>MGHQNAAVSENQNHDDGAASSPGFKLVGFSKFVRKNPKSDKFKVKRFHHIEFWCGDATNVARRFSWGLGMRFSAKSDLSTGNMVHASYLLTSGDLRFLFTAPYSPSLSAGEIKPTTTASIPSFDHGSCRSFFSSHGLGVRAVAIEVEDAESAFSISVANGAIPSSPPIVLNEAVTIAEVKLYGDVVLRYVSYKAEDTEKSEFLPGFERVEDASSFPLDYGIRRLDHAVGNVPELGPALTYVAGFTGFHQFAEFTADDVGTAESGLNSAVLASNDEMVLLPINEPVHGTKRKSQIQTYLEHNEGAGLQHLALMSEDIFRTLREMRKRSSIGGFDFMPSPPPTYYQNLKKRVGDVLSDDQIKECEELGILVDRDDQ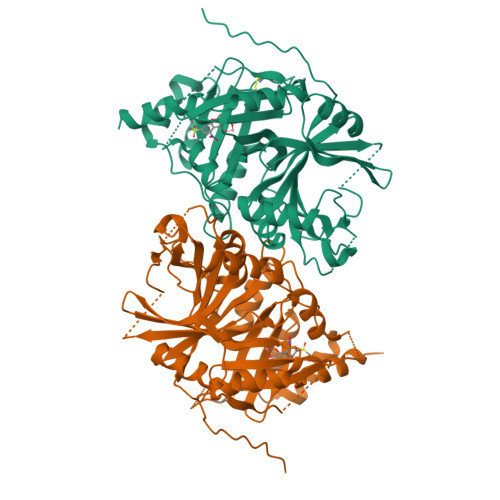GTLLQIFTKPLGDRPTIFIEIIQRVGCMMKDEEGKAYQSGGCGGFGKGNFSELFKSIEEYEKTLEAKQLVG[2x]>GAMPDGG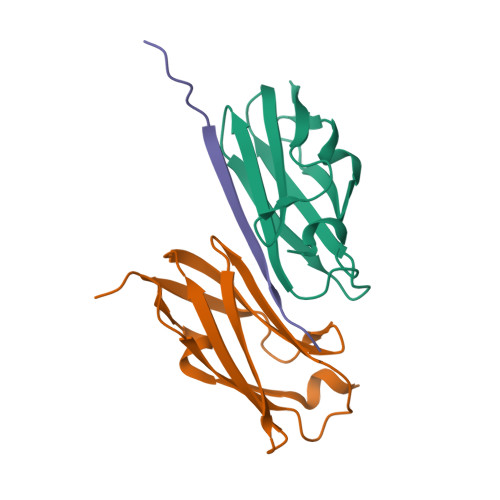AHKVRAGGPGLERAEAGVPAEFSIWTREAGAGGLAIAVEGPSKAEISFEDRKDGSCGVAYVVQEPGDYEVSVKFNEEHIPDSPFVVPVASPS[2x];> PLEKASVVSKLFFSWTAP> MKESRAKKFQRQHMDSDSSPSSSSTYCNQMMRRRNMTQGRCKPVNTFVHEPLVDVQNVCFQEKVTCKNGQGNCYKSNSSMHITDCRLTNGSRYPNCAYRTSPKERHIIVACEGSP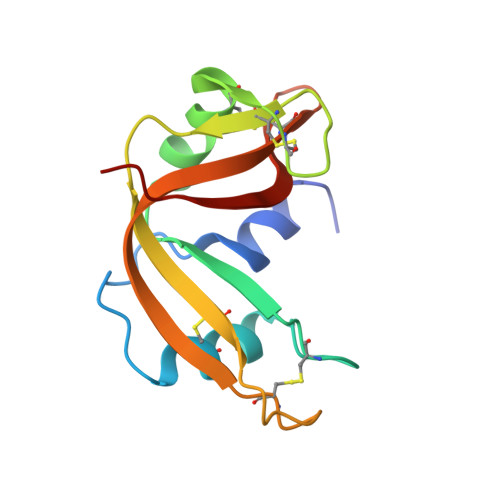YVPVHFDASVEDST> MSNEYNPPLGIAFRLCGLASDRVLFS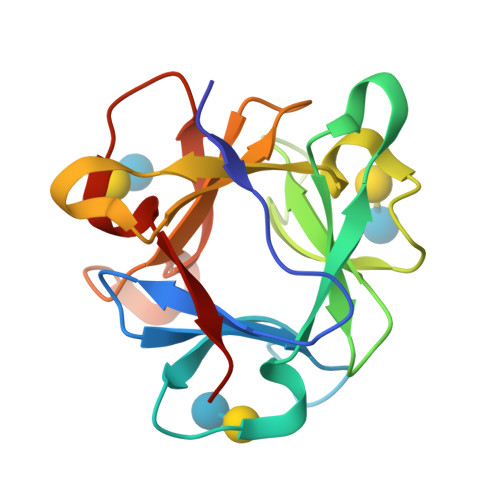RVSPSPEVFHHPKSEVYPDQWFVAIPGSGQNAGCYAIKSKNTGKVLFSRMSPDPRVGHIDGDGKYPDNWFKFEAGSGKYAGYFRLRAVASDTVLVSRTSTGTDTQVINYPATSAKYDDQYFTILFD> GPLGSMKQMGSMHPVQVIAVTGGKGGVGKTNVSVNLALALADLGRRVMLLDADLGLANVDVLLGLTPKRTLADVIEGRCELRDVLLLGPGGVRIVPAASGTQSMVHLSPMQHAGLIQAFSDISDNLDVLVVDTAAGIGDSVVSFVRAAQEVLLVVCDEPTSITDAYALIKLLNRDHGMTRFRVLANMAHSPQEGRNLFAKLTKVTDRFLDVALQYVGVIPYDESVRKAVQKQRAVYEAFPRSKASLAFKAVAQKVDSWPLP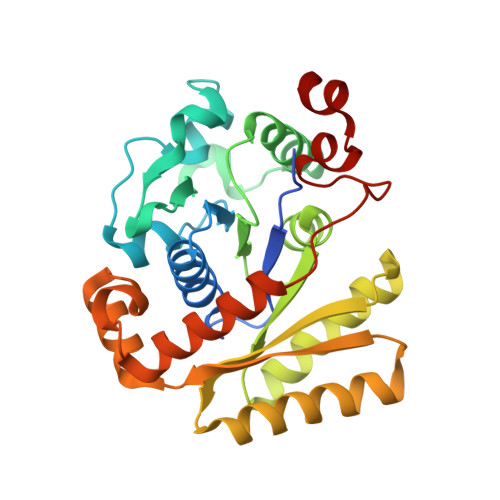ANPRGHLEFFVERLVQHPATGSAV(2S)-2,3-DICHLOROPROPAN-1-OL | C3 H6 Cl2 O | 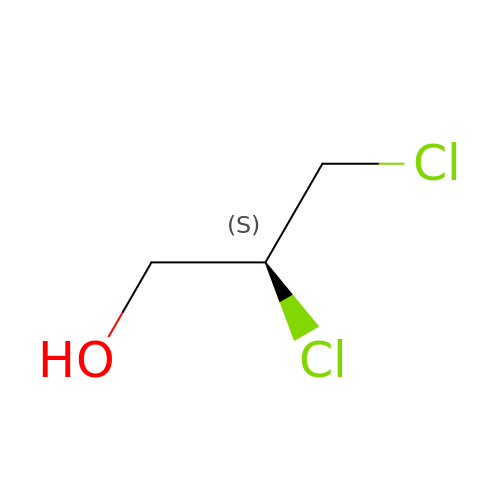ZXCYIJGIGSDJQQ-GSVOUGTGSA-N>[3x]MSTVVVKGNVNGGVQQPRMRRRQSLRRRANRVQPVVMVTAPGQPRRRRRRRGGNRRSRRTGVPRGRGSSETFVFTKDNLVGNTQGSFTFGPSLSDCPAFKDGILKAYHEYKIT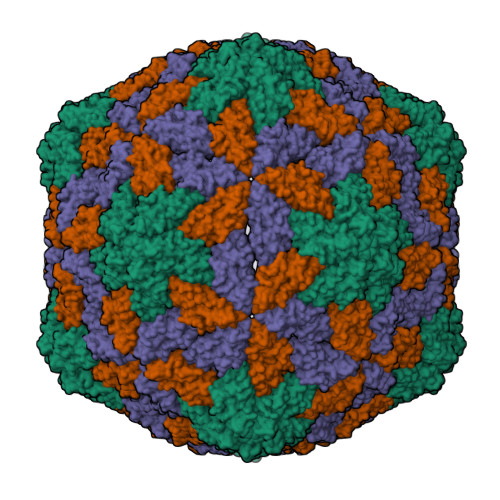SILLQFVSEASSTSSGSIAYELDPHCKVSSLQSYVNKFQITKGGAKTYQARMINGVEWHDSSEDQCRILWKGNGKSSDSAGSFRVTIKVALQNPK>[3x]MRCIGISNRDFVEGVSGGSWVDIVLEHGSCVTTMAKNKPTLDFELIKTEAKHPATLRKYCIEAKLTNTTTASRCPTQGEPSLNEEQDKRFVCKHSMVDRGWGNGCGLFGKGGIVTCAMFTCKKNMEGKVVQPENLEYTIVITPHSGEENAVGNDTGKHGKEIKVTPQSSITEAELTGYGTVTMECSPRTGLDFNEMVLLQMENKAWLVHRQWFLDLPLPWLPGADTQGSNWIQKETLVTFKNPHAKKQDVVVLGSQEGAMHTALTGATEIQMSSGNLLFTGHLKCRLRMDKLQLKGMSYSMCTGKFKVVKEIAETQHGTIVIRVQYEGDGSPCKIPFEIMDLEK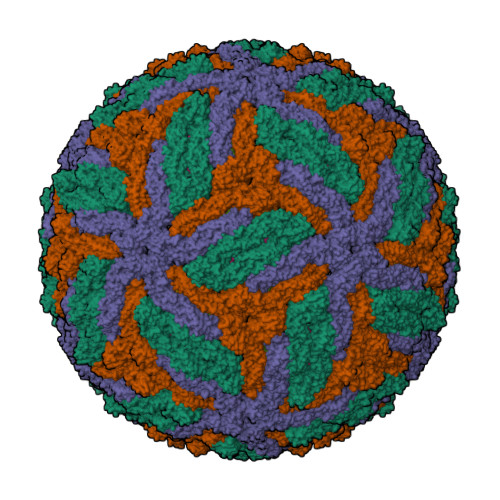RHVLGRLITVNPIVTEKDSPVNIEAEPPFGDSYIIIGVEPGQLKLSWFKKGSSIGQMFETTMRGAKRMAILGDTAWDFGSLGGVFTSIGKALHQVFGAIYGAAFSGVSWTMKILIGVVITWIGMNSRSTSLSVSLVLVGVVTLYLGVMVQA;>[3x]SVALVPHVGMGLETRTETWMSSEGAWKHAQRIETWVLRHPGFTIMAAILAYTIGTTYFQRVLIFILLTAVAPSMT> GPLGSARLRKLRKKEAKQRWDDRHWSQKKLDEMTDRDWRIFREDYSITTKGGKIPNPIRSWKDSSLPPHILEVIDKCGYKEPTPIQRQAIPIGLQNRDIIGVAETGSGKTAAFLIPLLVWITTLPKIDRIEESDQGPYAIILAPTRELAQQIEEETIKFGKPLGIRTVAVIGGISREDQGFRLRMGCEIVIATPGRLIDVLENRYLVLSRCTYVVLDEADRMIDMGFEPDVQKILEHMPVSNQKPDTDEAEDPEKMLANFESGKHKYRQTVMFTATMPPAVERLARSYLRRPAVVYIGSAGKPHERVEQKVFLMSESEKRKKLLAILEQGFDPPIIIFVNQKKGCDVLAKSLEKMGYNACTLHGGKGQEQREFALSNLKAGAKDILVATDVAGRGIDIQDVSMVVNYDMAKNIEDYIHRIGRTGRAGKSGVAITFLTKEDSAVFYELKQAILESPVSSCPPELANHPDAQHKPGTILTKKRREETIFA

The DEAD-box protein Prp28 is essential for pre-mRNA splicing as it plays a key role in the formation of an active spliceosome. Prp28 participates in the release of the U1 snRNP from the 5′-splice site during association of the U5·U4/U6 tri-snRNP, which is a crucial step in the transition from a pre-catalytic spliceosome to an activated spliceosome. Human Prp28 (hPrp28; also denoted U5-100K) comprises 820 amino-acid residues. The helicase core with the conserved sequence motifs corresponds to the C-terminal half of the protein.

Here, we report the crystal structure of hPrp28ΔN, a fragment of human Prp28 comprising the entire helicase core and a short N-terminal extension (NTE). The structure was refined at a resolution of 2.0 Å and contains residues 352–806. The three-dimensional structure of hPrp28ΔN can be divided into four parts: an N-terminal extension (NTE; residues 352–378), the N-terminal RecA-like domain (RecA-1; residues 379–629), the linker region (residues 630–639) and the C-terminal RecA-like domain (RecA-2; residues 640–806). In the crystal the helicase domain adopts a wide-open conformation, as the two RecA-like domains are extraordinarily displaced from the productive ATPase conformation. Interestingly, the defined arrangement of the hPrp28ΔN RecA domains appears to be a favourable one as there are many intramolecular contacts between the two RecA domains, e.g. a salt bridge between Lys382 and Glu640 and five hydrogen bonds (Ile379–Gly759, Thr381–Gly759, Thr381–Ser761, Lys382–Val788 and Glu614–Ser790). Interestingly, the linker of Prp28 appears to be arrested in its conformation by a tight network of hydrogen bonds, which consequently keeps the RecA domains in a wide-open state. A unique feature of hPrp28 is the insertion of 24 amino acids (residues 576–599), which form a protuberance on the RecA-1 domain. Binding of ATP is hindered by a closed conformation of the P-loop, which occupies the space required for the γ-phosphate of ATP. Moreover, the conformation of the P-loop is affected by the bound sulfate ion located between the proposed binding sites of the α- and β-phosphates of the ATP.>MADVTGIALGMIETRGLVPAIEAADAMTKAAEVRLVGRQFVGGGYVTVLVRGETGAVNAAVRAGADACERVGDGLVAAHIIARVHSEVENILPKAPQA[8x];> MKIMQVEKTLVSTNRIADMGHKPLLVVWEKPGAPRQVAVDAIGCIPGDWVLCVGSSAAREAAGSKSYPSDLTIIGIIDQWNGE;> MNPADLSGLSGKELARARRAALSKQGKAAVSNKTASVNRSTKQAASSINTNQVRSSVNEVPTDYQMADQLCSTIDHADFGTESNRVRDLCRQRREALSTIGKKAVKTNGKPSGRVRPQQSVVHNDAMIENAGDTNQSSSTSLNNELSEICSIADDMPERFGSQAKTVRDICRARRQALSERGTRAVPPKPQSQGGPGRNGYQIDGYLDTALHGRDAAKRHREMLCQYGRGTAPSCKPTGRVKNSVQSGNAAPKKVETGHTLSGGSVTGTQVDRKSHVTGNEPGTCRAVTGTEYVGTEQFTSFCNTSPKPNATKVNVTTTARGRPVSGTEVSRTEKVTGNESGVCRNV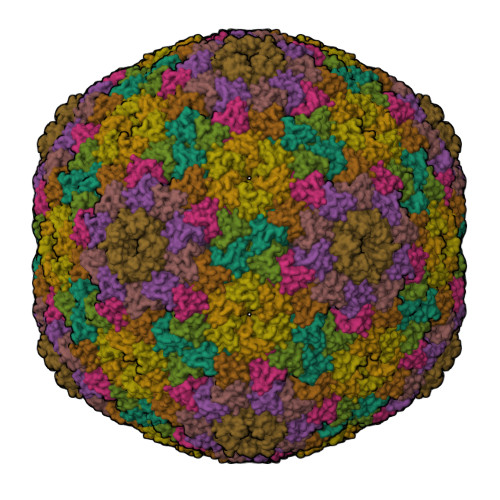TGTEYMSNEAHFSLCGTAAKPSQADKVMFGATARTHQVVSGSDEFRPSSVTGNESGAKRTITGSQYADEGLARLTINGAPAKVARTHTFAGSDVTGTEIGRSTRVTGDESGSCRSISGTEYLSNEQFQSFCDTKPQRSPFKVGQDRTNKGQSVTGNLVDRSELVTGNEPGSCSRVTGSQYGQSKICGGGVGKVRSMRTLRGTSVSGQQLDHAPKMSGDERGGCMPVTGNEYYGREHFEPFCTSTPEPEAQSTEQSLTCEGQIISGTSVDASDLVTGNEIGEQQLISGDAYVGAQQTGCLPTSPRFNQTGNVQSMGFKNTNQPEQNFAPGEVMPTDFSIQTPARSAQNRITGNDIAPSGRITGPGMLATGLITGTPEFRHAARELVGSPQPMAMAMANRNKAAQAPVVQPEVVATQEKPELVCAPRSDQMDRVSGEGKERCHITGDDWSVNKHITGTAGQWASGRNPSMRGNARVVETSAFANRNVPKPEKPGSKITGSSGNDTQGSLITYSGGARG>GDELQETSKEATNFSISIDDALSDPLTRTSNDLFPARNSITTGEVISMAASGQDYTPFIVGKDSRAWNEIGTATGTVTFYAHYPALTDEAATRSGGNKRYLKGGQEHLFGTAEAAPGSQNVSLKFKRMTVPVIILDE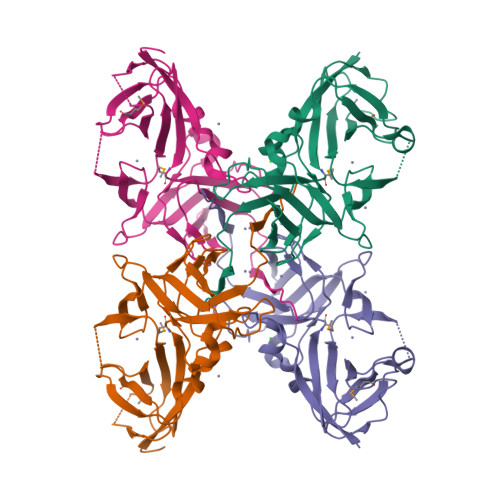NDRPYEGEAKVELSLKNEGTQDLLNGTIEINENALSENIEVKKVSEGVTTNVLPQKINAGEEIGTITVGGVTQKISAVEDLDLKAGSTLSVRLSKKFGGGIIDGNVPLYR[2x]> RSPWNRIPESGGDNSVFDIFELTGAARKGSGRRLVKGPDPSSPAFRIEDANLIPPVPDDKFQDLVDAVRTEKGFLLLASLRQMKKTRGTLLALERKDHSGQVFSVVSNGKAGTLDLSLTVQGKQHVVSVEEALLATGQWKSITLFVQEDRAQLYIDCEKMENAELDVPIQSVFTRDLASIARLRIAKGG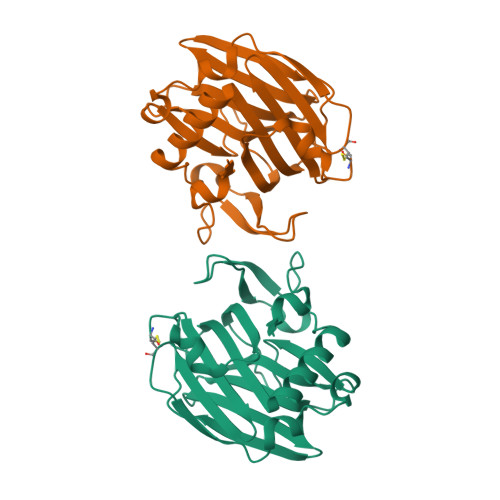VNDNFQGVLQNVRFVFGTTPEDILRNKGCSSSTSVLLTLDNNVVNGSSPAIRTNTGHHHHHH>MKYGIVLFPSKKLQDLANSYRKRYDPSYSLIPPHLTLRASFECAE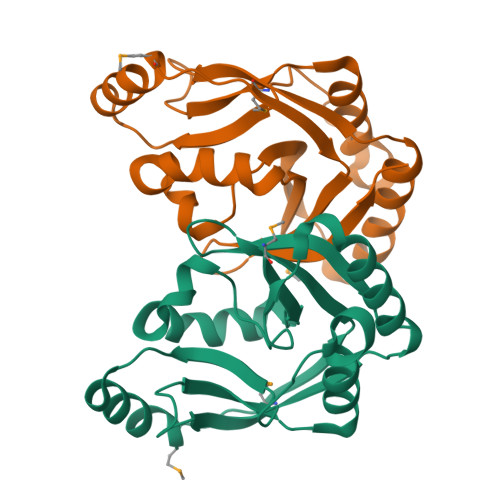EKADQLVSHLRNIAKESHPLVLKMTKYSSFAPVNNVIYIKAEPTEELKTLNEKLYTGVLAGEQEYNFVPHVTVGQNLSDDEHSDVLGQLKMQEVSHEEIVDRFHLLYQLENGSWTVYETFLLGRGE[2x]> MANKESELNGLDDIHSDIEKLSAHVEKFSDGMDEKYKELTARFDGVKGDNDAIRKAVADATKEYAELSAKHQFFTEELAAMKARLDTPIMRSQAELDDHDRKTAIQLQRNMHEFRGGDPKEFVADESNLVDLKAYRSAVRKMLKVGIESKERVIASMTDVERKAFEASTIGPAFFTPQVLALEVDCNIECASLLDL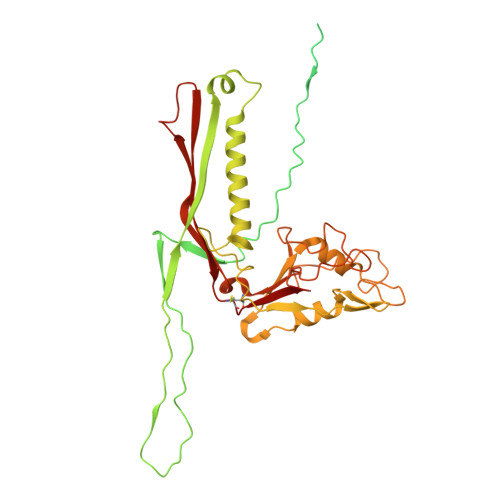YGQIEVSRSTFTYMKIADYGQLGEYTCDAKCDAEFGEPGNIRHLEGKTYDYRGVFCFNRKNLQEANYDFLSFMIGAAQRSHRINRNQALMIGKGVNEPKGWLTENCFPVFQTLPVDVNGTSTPAFLAQDWRRFVTSFPAEYGEARSVMHQNVFGYLAAMVDANGRFLFGDGDLTFTPDLVRERIRISNCLPDPTEGNTKGGTGQDAFAAGSFVAAQAAWKTAFYAVEKRPMFFEQYEGGSSAWCVKYQFGAEDGGFVGCCEHGRILQIG>GNNRALINDKLASLQYNPKTVMVFNGTSISNIDLPAEERFDDSTYIVMTREKCSYEADFDIAVPSAYEDVTYPGALLVASNDLLDGKPQELAVDKDRVNITVDLPGATDISFKVVPTFANVRAGINDILSKWFDSHGGEWSLPANFQYSSSLVYDENELMLKFGCDISYLKQKLSIDFSSTRAEKKSVYLIRFKQIFYSVSAERPAKPADIFAESTTWEDLARAGISEEHPPLFVKNVQYGRQIFLKFESKLSSTELETTIKGTCSKDGLKIDANASAALKEKLSQIDVSIVVHGGSEAVYNGLSLNSMDDVQKINRIIWDNTLLSRTNTAAPLNYYTVFLKDGVSAGVHGTTEYVAEKTERYSGGEIRLEHSGWYVARFTVTWDEISYENGLKVIRHKGWEGNGKDRTAPFSTTIPLRGNARNISIKTEGCTGLAWEWWRTSGYKVGRALVPLRTVSIGGTTLHQTFSMTPAD[2x]

The cholesterol-dependent cytolysin (CDC) genes are present in bacterial species that span terrestrial, vertebrate, and invertebrate niches, which suggests that they have evolved to function under widely different environmental conditions. The study of the pore-forming mechanism of the cholesterol-dependent cytolysins (CDCs) has established paradigms that have served as a basis for understanding the mechanisms of a wide array of pore-forming proteins (1), including the membrane attack complex/perforin-like (MACPF) proteins (2) and the stonefish family of venom toxins (SNTX) (3). These proteins all exhibit an analogous protein fold to domain 3 (D3) of the CDCs, which forms the β-barrel pore. The disruption of this interface allows the formation of the membrane spanning β-barrel pore in all CDCs.

We further show that the CDC from the terrestrial bacterium D. propionicus (desulfolysin [DLY]), unlike PFO, exhibits a high level of pore-forming activity across a wide spectrum of temperatures. DLY was crystallized, and its structure was determined by multiple anomalous dispersion to a resolution of 2.3 Å. Despite the relatively low sequence homology between DLY and CDCs from Gram-positive bacteria (∼40% identity with PFO) with known crystal structures, DLY adopts a similar overall shape, topology, and domain arrangement. Most CDCs have just one cysteine residue, which is located in the undecapeptide motif, whereas DLY has three additional cysteine residues (C54 in D2 and C166 and C266 in D3), none of which are in a disulfide, although C166 could not be altered without decreasing pore-forming activity (E. M. Hotze and R. K. Tweten, unpublished data; also reference 4). The D3-D1,2 interface in DLY differs substantially from that in PFO. There are fewer than half as many D3-D1,2 interfacial water molecules identifiable in the crystal structure of DLY, compared to PFO (15 and 37, respectively), which can be attributed, in part, to the greater number of bulky nonpolar residues that result in a more tightly packed interface that excludes solvent. In DLY, 49% of the interfacial residues are nonpolar compared to 38% in PFO, and to a large extent, the nonpolar residues in PFO are not in complementary interactions (i.e., hydrophobic-hydrophobic), whereas they are in DLY. Consequently, there is a greatly reduced number of hydrogen bonding interactions present across the interface, with 12 protein-to-protein H-bonds in PFO compared to only 6 in DLY. Interestingly, the analogous loop in native DLY (S66 to P74) adopts a conformation similar to that observed in PFON197W where it does not contact the glycine pair analogue (G296, G297) in DLY. One significant difference in the D3-D1,2 interface with that of PFO is the presence of a strong nonpolar interaction between the side chain of L162 in αHB1 (which refolds into transmembrane β-hairpin 1) and a hydrophobic core of D2 residues consisting of F25, Y56, A58, and F60.> NQDGQLVEQEVRRLLATAAYKDVVLTSPKEGEPWLLTGYIQDNHARLSLQNFLESHGIPFRLELRSMEELRQGAEFILQRLGYHGIEVSLAPQAGWLQLNGEVSEEIQKQKIDSLLQAEVPGLLGVENKVRIAPNQRKRLDALLEQFGLDSDFTVNVKGELIELRGQVNDEKLSSFNQLQQTFRQEFGNRPKLELVNV

acts as a connector between the secretin and the IM (YscD, PrgH, MxiG). YscD is known to have four periplasmic domains.

* indicates the junction between YscC and YscD. to Y. enterocolitica injectisomes by YscC and YscD. about the interaction between the YscD and YscJ protomers. YscD units would lead to a poorer match with the experimental data. the YscJ 24-mer further supports the proposed stoichiometry. forcing a preferential perpendicular orientation to the IM. confirming the preferential orientation found in the 24-mer YscD ring assembly. YscDJ ring modeling has been performed to test for any elasticity of the basal body.>VQRGYGNPIEASSYGLDLDCGAPGTPEAHVCFDPCQNYTLLDEPFRSTENSAGSQGCDKNMSGWYRFVGEGGVRMSETCVQVHRCQTDAPMWLNGTHPALGDGITNHTACAHWSGNCCFWKTEVLVKACPGGYHVYRLEGTPWCNLRYCTDPSHHHHHHHH[2x]

Glycoprotein 2 (GP2) and uromodulin (UMOD) filaments protect against gastrointestinal and urinary tract infections by acting as decoys for bacterial fimbrial lectin FimH. By combining AlphaFold2 predictions with X-ray crystallography and cryo-EM, we show that these proteins contain a bipartite decoy module whose new fold presents the high-mannose glycan recognized by FimH. The structure rationalizes UMOD mutations associated with kidney diseases and visualizes a key epitope implicated in cast nephropathy.

To address these questions, we first expressed in mammalian cells the whole GP2 branch as well as the corresponding region of UMOD and assessed their ability to selectively capture the lectin domain of FimH (FimHL) from an Escherichia coli periplasmic extract. This showed that, as in the case of UMOD, the branch of GP2 is sufficient for interaction with FimHL. We then obtained crystals of the GP2 branch, but experimental phasing of its 1.9-Å-resolution data was hindered by relatively high diffraction disorder in one direction and low crystal symmetry. The electron density maps reveal that the GP2 branch is a protein module (henceforth referred to as ‘decoy module’) that consists of a β-hairpin stabilized by a disulfide bond (Cx48-Cy59), packed against a globular ‘D10C’ domain with a new fold including two 310 helices, nine β-strands (βA–βI) and five intermolecular disulfides (C163-C8157, C285-C9172, C3107-C6145, C4113-C10177, C5138-C7146). Interestingly, although the GP2 branch also binds FimHL, its D10C domain cannot be glycosylated at the position corresponding to UMOD N275 (R165). In agreement with these considerations, introduction of an N65A mutation in the decoy module of GP2 impairs its interaction with FimHL and mass spectrometric analysis of the glycans attached to N65 detects the HexNAc2Hex5 oligomannose structure, indicating that UMOD and GP2 exploit a common molecular strategy to counteract bacterial adhesion. Because of 60% sequence identity to UMOD, the crystal structure of the latter immediately explains the effect of many substitutions affecting invariant positions. Remarkably, most of these mutations cluster within two structurally important regions of the decoy module, the β-hairpin/D10C domain groove and the disulfide bond-rich region at the opposite end of D10C.>MAHHHHHHHHHHKLTSLYKKAGLENLYFQGLAADEGADDAVAAEEERDLDALPASYADWQRRLRATTDEARPAAVEKRHAAGKLTARENVAALLDAGSFNEHGALALAAQRGRRSEEELLALSPADGLITGVGTVNAGQFPDTAACAVAAYDYTVLAGTQGYFNHHKLDRLIALAGQWKWPLVLFAEGGGGRPGDTDMPVAAALVTPTFLNFAALSGQVPLVGVAAGACFAGNAALLGCCDVVIATRDSSIGLGGPAMIEGGGLGVVAAGDIGPAEVLAQKGVVDLLAENDAEANELARRYLTYFQGDVTGWEAADQRELRWVIPQVRKRAYDVRALLHLLADTGSVLELRRAFAPGLLTALVRIGGKAFGVIANDPAVLGGAIDAAGADKAARFLNLCDTHRLPVLSLVDTPGFMVGPASEAEGAVRHVSRLFVRAAKLTVPFFA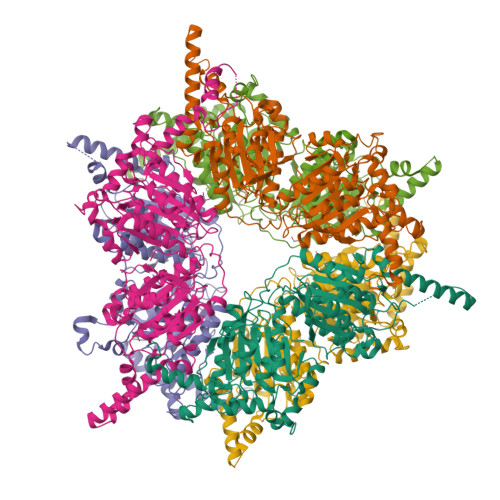VVTRRAYGLGAQAMAAGSLHAPALTVSWPGGEFGPMGLEGAVRLGYRRELAAVSDPQEREALYQKLVAQAYAQGEAVNVAAHLEVDAVIDPAETRNWLLRALRVSPYSAQRREGGLVDPW[6x]>[8x]MNLIKEDMRVKVHMEGNVNG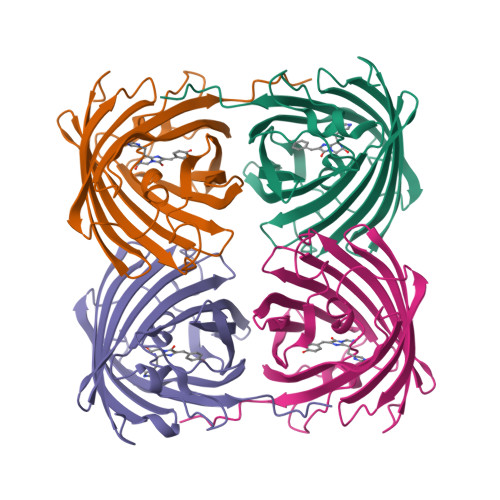HAFVIEGEGKGKPYEGTQTLNLTVKEGAPLPFSYDILTTALHYGNRVFTKYPEDIPDYFKQSFPEGYSWERTMTYEDKGICTIRSDISLEGDCFFQNVRFNGMNFPPNGPVMQKKTLKWEPSTEKLHVRDGLLVGNINMALLLEGGGHYLCDFKTTYKAKKVVQLPDYHFVDHRIEILSNDSDYNKVKLYEHGVARYSPLPSQAW> GTRDRDSQRDLVEAVAHILGIRDLAAV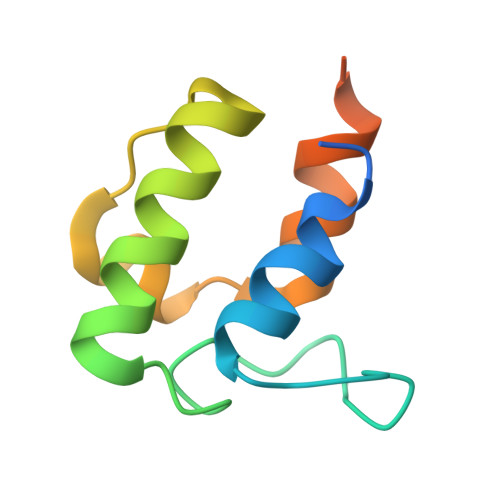NLDSSLADLGLDALMSVEVRQTLERELNLVLSVREVRQLTLRKLQELSSKADEASELACPTPKE> NDPITNAVESAVSALADTTISRVTAANTAASTHSLGTGRVPALQAAETGASSNSSDENLIETRCVMNRNGVNEASVEHFYS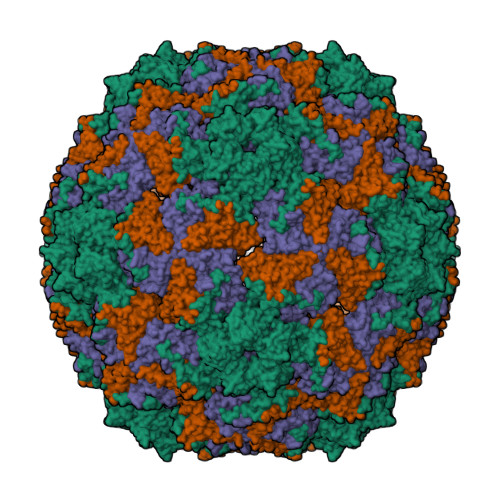RAGLVGVVEVKDSGTSLDGYTVWPIDVMGFVQQRRKLELSTYMRFDAEFTFVSNLNNSTTPGMLLQYMYVPPGAPKPDSRKSYQWQTATNPSVFAKLSDPPPQVSVPFMSPATAYQWFYDGYPTFGEHKQATNLQYGQCPNNMMGHFAIRTVSESTTGKNIHVRVYMRIKHVRAWVPRPLRSQAYMVKNYPTYSQTITNTATDRASITTTDYEGGVPASPQRTS;> SPSVEACGYSDRVAQLTVGNSTITTQEAANIVLSYGEWPEYCPSTDATAVDKPTRPDVSVNRFYTLSTKSWKTESTGWYWKFPDVLNDTGVFGQNAQFHYLYRSGFCMHVQCNASKFHQGALLVAAIPEFVIAASSPATKPNSQGLYPDFAHTNPGKDGQEFRDPYVLDAGIPLSQALIFPHQWINLRTNNCATIIMPYINALPFDSALNHSNFGLVVIPISPLKYCNGATTEVPITLTIAPLNSEFSGLRQAIKQ;> GFPTELKPGTNQFLTTDDGTSPPILPGFEPTPLIHIPGEFTSLLDLCQVETILEVNNTTGTTGVSRLLIPVRAQNNVDQLCASFQVDPGRNGPWQSTMVGQICRYYTQWSGSLKVTFMFTGSFMATGKMLIAYTPPGSAQPTTREAAMLGTHIVWDFGLQSSVTLVIPWISNTHFRAVKTGGVYDYYATGIVTIWYQTNFVVPPDTPTEANIIALGAAQKNFTLKLCKDTDEIQQTAEYQ> IVGGQECKDGECPWQALLINEENE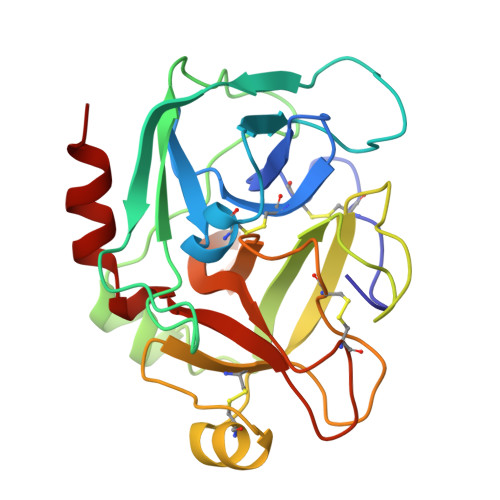GFCGGTILSEFYILTAAHCLYQAKRFKVRVGDRNTEQEEGGEAVHEVEVVIKHNRFTKETYDFDIAVLRLKTPITFRMNVAPACLPERDWAESTLMTQKTGIVSGFGRTHEKGRQSTRLKMLEVPYVDRNSCKLSSSFIITQNMFCAGYDTKQEDACQGDSGGPHVTRFKDTYFVTGIVSWGEGCARKGKYGIYTKVTAFLKWIDRSMKTR>TKAVTFYEDINYGGASVSLQPGNYTLSQLNTAKIPNDWMTSLKVPSGWTVDVYENDNFTGTKWTYTSDTPWVGNDANDKMTSVKIYST[8x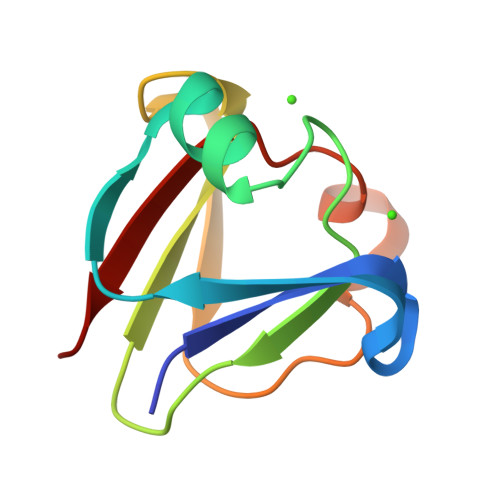]>ETGASAKELACQEITVPLCKGIGYEYTYMPNQFNHDTQDEAGLEVHQFWPLVEIQCSPDLKFFLCSMYTPICLEDYKKPLPPCRSVCE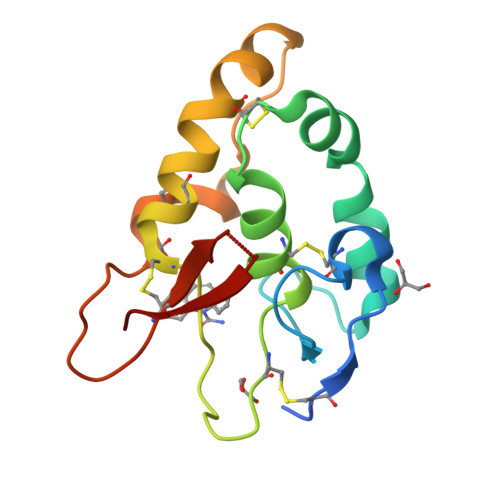RAKAGCAPLMRQYGFAWPDRMRCDRLPEQGNPDTLCMDYERGTLEVLFQG[2x]>[2x]AFADKPNHFINFPLAQFSGFMGKYLKLQSQLVEMGLDCK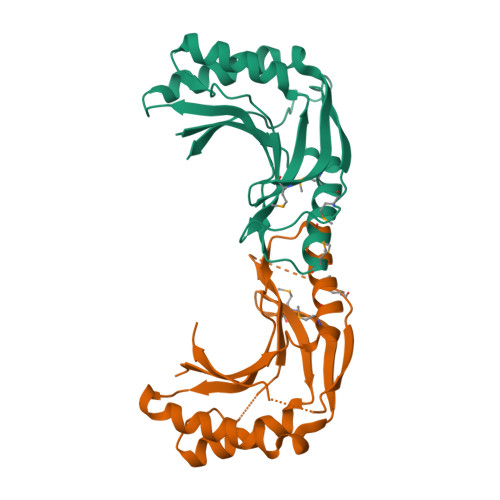LQKAPHVSITLLDIKADQYKQVEFAIQEIIDDLAAYEGDIVFDNPHMLGRCLVLDVRGFEELHEDIVEILRRRGCTADQSRHWIPHCTVAQFDEERETKGMQFYHKEPFYLKHNNLLTDAGLELVKIGSSKIDGFYCSELSVWCGERLCYKPPTPKFSDGSGSHHHHHH> DQAGKSPNAVRYHGGDEIILQGFHWNVVREAPNDWYNILRQQAATIAADGFSAIW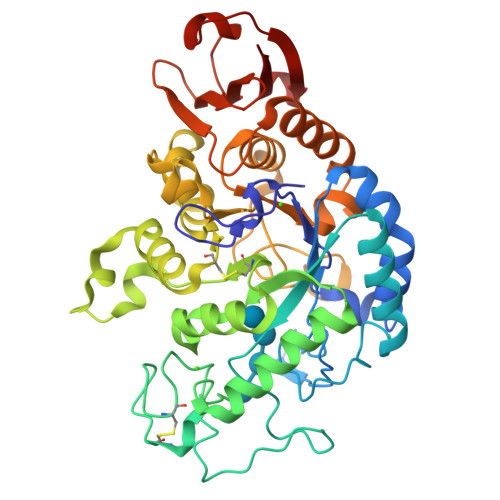MPVPWRDFSSWSDGSKSGGGEGYFWHDFNKNGRYGSDAQLRQAASALGGAGVKVLYDVVPNHMNRGYPDKEINLPAGQGFWRNDCADPGNYPNDCDDGDRFIGGDADLNTGHPQVYGMFRDEFTNLRSQYGAGGFRFGFVRGYAPERVNSWMTDSADNSFCVGELWKGPSEYPNWDWRNTASWQQIIKDWSDRAKCPVFDFALKERMQNGSIADWKHGLNGNPDPRWREVAVTFVDNHDTGYSPGQNGGQHHWALQDGLIRQAYAYILTSPGTPVVYWDHMYDWGYGDFIRQLIQVRRAAGVRADSAISFHSGYSGLVATVSGSQQTLVVALNSDLGNPGQVASGSFSEAVNASNGQVRVWRS> GRRRRLVWTPSQSEALRAC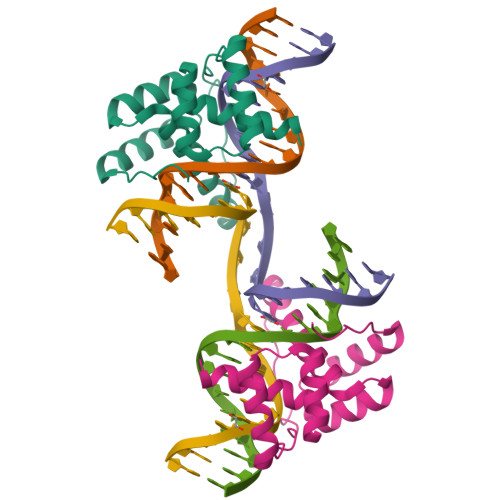FERNPYPGIATRERLAQAIGIPEPRVQIWFQNERSRQLRQHRRESRPWPGRRGPPEGRRKRTAVTGSQTALLLRAFEKDRFPGIAAREELARETGLPESRIQIWFQNRRARHP>GSHMASSRNYLKNPGFETGEFSPWRVSGDKKAVKVVKANPSSNAHQGEYAVNFWLDESFSFELSQEVELPAGVYRVGFWTHGEKGVKIALKVSDYGGNERSVEVETTGWLEWKNPEIRNIKVETGRIKITVSVEGRAGDWGFIDDFYLFREE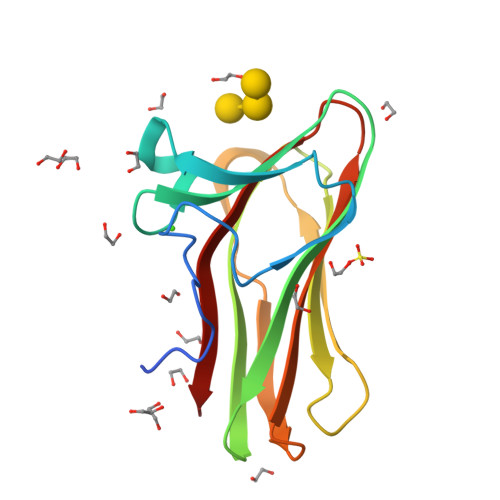[2x]> DVVRASRNAKVKGKFRESYLSPAQSVKPKINTEEKLPREKLNPPTPSIYLESKRDAFSPVLLQFCTDPRNPITVIRGLAGSLRLNLGLFSTKTLVEASGEHTVEVRTQVQQPSDENWDLTGTRQIWPCESSRSHTTIAKYAQYQASSFQESLQEEKESEDEESEEPDSTTGTPPSSAPDPKNHHIIKFGTNIDLSDAKRWKPQLQELLKLPAFMRVTSTGNMLSHVGHTILGMNTVQLYMKVPGSRTPGHQENNNFCSVNINIGPGDCEWFAVHEHYWETISAFCDRHGVDYLTGSWWPILDDLYASNIPVYRFVQRPGDLVWINAGTVHWVQATGWCNNIAWN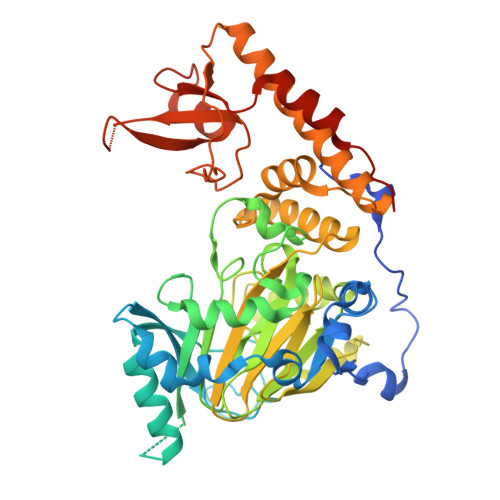VGPLTAYQYQLALERYEWNEVKNVKSIVPMIHVSWNVARTVKISDPDLFKMIKFCLLQSMKHCQVQRESLVRAGKKIAYQGRVKDEPAYYCNECDVEVFNILFVTSENGSRNTYLVHCEGCARRRSAGLQGVVVLEQYRTEELAQAYDAFTLAPASTSRHHHHHH>MKHHHHHH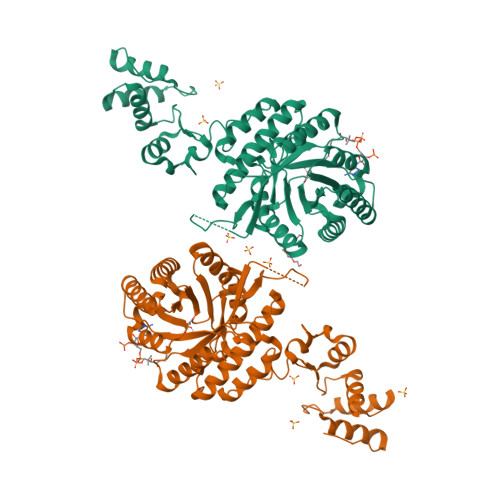HHGGLVPRGSHGGSMLPKKKLHMKVGILDSTLREGEQTPGVVFTTDQRVEIAKALSDIGVQMIEAGHPAVSPDIYEGIRRIIKLKREGVIKSEIVAHSRAVKRDIEVGAEIEADRIAIFYGISDTHLKAKHHTTRDEALRSIAETVSYAKSHGVKVRFTAEDATRADYQYLLEVIKTVRDAGADRVSIADTVGVLYPSRTRELFKDLTSRFPDIEFDIHAHNDLGMAVANVLAAAEGGATIIHTTLNGLGERVGIAPLQVVAAALKYHFGIEVVDLKKLSEVASLVEKYSGIALPPNFPITGDYAFVHKAGVHVAGVLNDPKTYEFLPPETFGRSRDYVIDKYTGKHAVKDRFDRLGVKLTDSEIDQVLAKIKSNPNVRFYRDVDLLELAESVTGRLEHHHHHH[2x]> TDSFLLRFLRARDFDLDLAWRLLKNYYKWRAECPEISADLHPRSIIGLLKAGYHGVLRSRDPTGSKVLIYRIAHWDPKVFTAYDVFRVSLI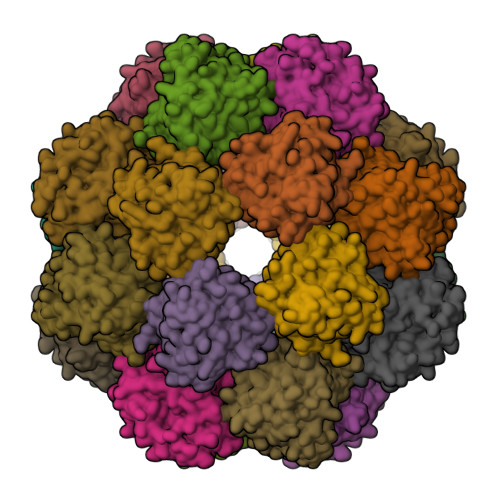TSELIVQEVETQRNGIKAIFDLEGWQFSHAFQITPSVAKKIAAVLTDSFPLKVRGIHLINEPVIFHAVFSMIKPFLTEKIKERIHMHGNNYKQSLLQHFPDILPLEYGGEEFSMEDICQEWTNFIMKSEDYLSSISESIQ>ETGYENTWNLYYEPPCCTGSSAAHHLRHHKEHVQDFSCGPLHYKTFYMDERNNALYVGAMDRIFRLNLRNISQSICERDVLILEPTGSDILNCVSKGKREKVECRNHIRVIQPMNFNGQKLYVCGTNAHNPKDYVINANLTHLPRSQYVPGIGLGIGKCPYDPADNSTAVYVENGNPFGLPALYAGTNAEFTKADSVIFRSDLYNLTNGRKEANFKRTVKYDSKLLDKPNFVGSFEIGEFVYFFFREHAVEYINCGKAVYSRVARVCKNDRGGKYMISQNWATYLKARMNCSISSEFPFYFNEIQSVYKMPTDDTKFYATFTTNTNGLIGSAVCSYDIRDINAAFDGKFKEQATSNSAWLPVLNSKVPEPRPGTCHNDTATLPDSVLNFIRKHPLMDKAVDHEFGNPVFFKRDVILTKLVVDKIRIDKLNQEFLVYFVATTSGHIYKIVQFMHYGQRHSNLVDIFEASPHSEPIREMTLSHKTGSLYVATDHQVKQIDIAMCARRYDSCFRCVSDPYCGWDKDVNACRPYQLGLLQDVANETSGICDTS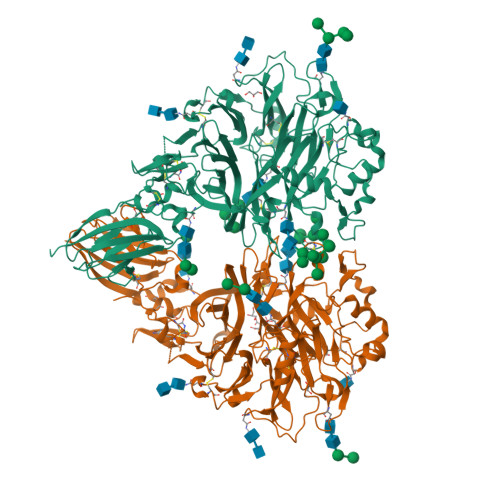VLRKKVTSSYGQTLHLSCFVKMPEVLRKKQTRWYHHSTEKGRYEVRYTPTKYIDTNEGGLVLLAVNEGDGGRYDSYLDGTLLCSYGVTVDAHRCSPPSQGTKHHHHHH[2x]>MRRTTKETDIIVEIGKKGEIKTNDLILDHMLTAFAFYLGKDMRITATYDLRHHLWEDIGITLGEALRENLPEKFTRFGNAIMPMDDALVLVSVDISNRPYANVDVNIKDAEEGFAVSLLKEFVWGLARGLRATIHIKQLSGENAHHIVEAAFKGLGMALRVATKESERVESTKG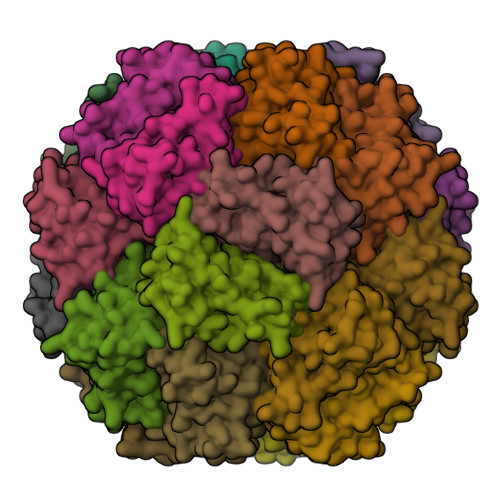VL[3x]> MVMLHSKNVKGFLENTLKPYDLHSVDFKTSSLQSSMIITATNGGILSYATSNNDVPKNSINEINSVNNLKMMSLLIKDKWSEDENDTEEQHSNSCYPVEIDSFKTKIYTYEMEDLHTCVA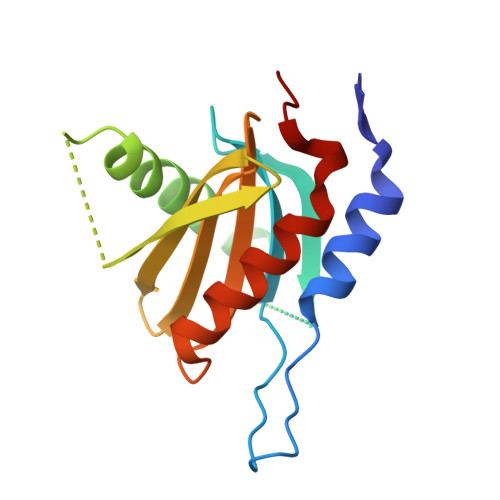QIPNSDLLLLFIAEGSFPYGLLVIKIERAMRELTDLFGYKLG>GAMGSGIQMKEEASEHGGSADETQELSPVSDSSDEMPNNAKRRRRSQSMIANKRIHQAFQEDEGDEDWEEEEHKPKAKRRYNTRSNESFSEGDDEPFEVSESSALEDELSDSEDSFIRSVRSKPKYKPGTRRSTRLRNRRSQDEEESEEEHRPILRERTSRINYSVPLAFPPVDEMDGDPSSQVNQSRSRKTHSELAITKLLRQQVSSFMPYIDSSGSESESDNTRIKKSSAKTIKALTDPANSGGPPDFGRIREKSDLADSDPLGVDSSLSFESVGGLDNYINQLKEMVMLPLLYPEIFQRFNMQPPRGVLFHGPPGTGKTLMARALAAACSSENKKVSFYMRKGADCLSKWVGEAERQLRLLFEEAKSTQPSIIFFDEIDGLAPVRSSKQEQIHASIVSTLLALMDGMESRGQVIIIGATNRPDAVDPALRRPGRFDREFYFPLPDRDARKKIIEIHTRNWDPPVPEWLCSMLAEKSKGYGGADLRALCTEAALNSIKRTYPQLYRSTKRLQIDPKTIKVKVKDFVMSMKRMIPSSERSSISPSKPLSPELKPLLNEAFQDIEKTLQKLMPVASKLNPLEEVMYDDPKENDFEYQQRLETFETLRIYKPRFLICGRKGLGQTALGPAILQQYEGVHVQSFDMSTLLQDSTQSIETSIIHLFLEVRRHTPSIIYIPDIDNWLNVLPLTAITTFSSMLERLDFSDQILFLALSSSPLSELHPQLREWFSSKQSVYSLQYPTRDSIIAFFQPILELIKASPTELPGGIPRKRRVLPELPLAPDPPPFTSQKITLKQTKQADMRLLNKLKIKLNALLGSLRARYRKFKKPLIDFNDIYCVDPETGHSYRSREECHYEFVDDVVKQIGSDQKFSMMSLEEIEKRTWDNCYCTPKQFVHDIKLILRDALQLEDSETIKRAQEMYANVLLGVEDMEDDQFSQRCERMALREAERRKLRHGKLQKHLDETKADMQ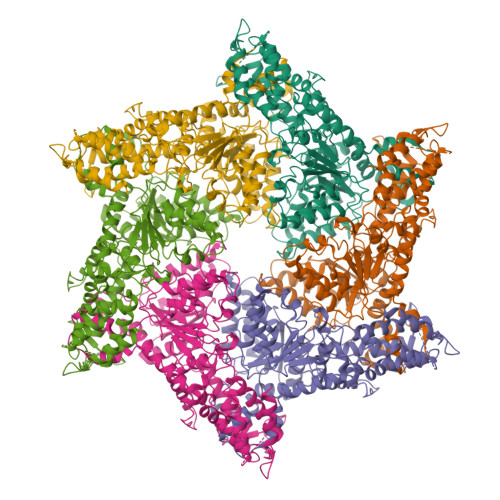FTSEKPSVDESITEVDDAIKDGPPVLAETLTNSLMEDVGPENVDMDIEDNEIFTNQSTMSVPSMLVENEESPKPDEYIDQKDKVQSPLLNGKSPVGVPSEAALRVSTDVSTNISSNGRADIPVDTLITSPADVPNNAPTDAHNITSADGHIENIEQEVVFPDLVFDEDRLTPLKQLLIDSTTGFTVDQLLHLHSFLYQIIWNTKSEWNRNSVVDECERAVKEFMINALQ[6x]Cytochalasin B | C29 H37 N O5 | 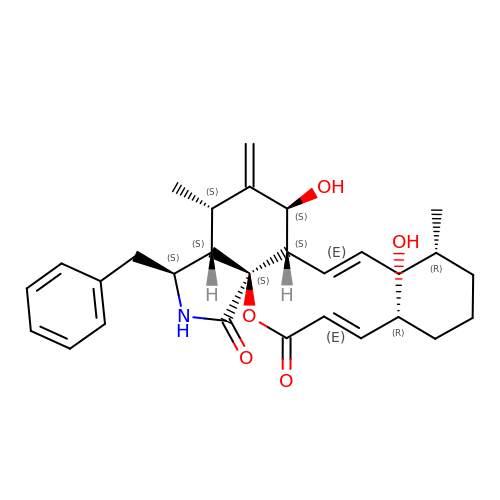GBOGMAARMMDZGR-TYHYBEHESA-N N-[(benzyloxy)carbonyl]-L-isoleucyl-L-leucine | C20 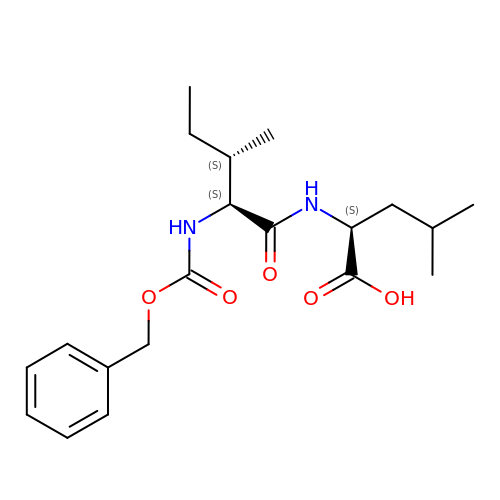H30 N2 O5 | BSRAGXJNZJMFMY-XIRDDKMYSA-N> MSLKIAAFGEVMLRFTPPEYLMLEQTEQLRMNFVGT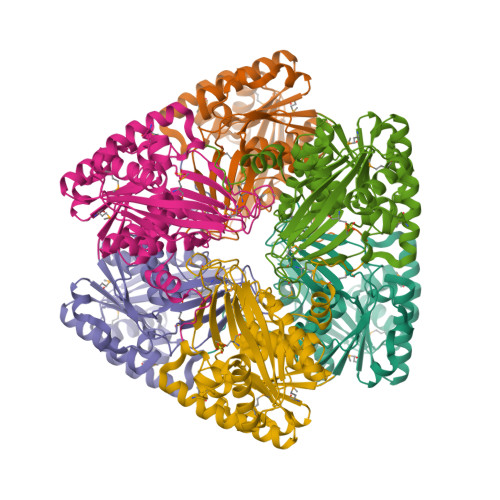GVNLLANLAHFQLETALITKLPANRLGEAGKAALRKLGISDQWVGEKGDHIGSFFAEMGYGIRPTQVTYQNRHQSAFGISEAKDYDFEAFLAEVDMVHICGISLSLTEKTRDAALILAQKAHAYQKKVCFDFNYRPSLNTANSALFMRQQYERILPYCDIVFGSRRDLVELLGFIPREDLEGEAQETELIQRFMSQYNLEWFAGTTRSHSQNQNYLSGYLYTQNEYQQSEKRPLLNLDRIGAGDAYAAGILYGYSQNWSLEKAVTFATVNGVLAHTIQGDIPLTTVKQVNHVLEHPNIDLIREGHHHHHH>PTYPKYLLSPETIEALRKPTFDVWLWEPNEMLSCLEHMYHDLGLVRDFSINPVTLRRWLFCVHDNYRNNPFHNFRHCFCVAQMMYSMVWLCSLQEKFSQTDILILMTAAICHDLDHPGYNNTYQINARTELAVRYNDISPLENHHCAVAFQILAEPECNIFSNIPPDGFKQIRQGMITLILATDMARHAEIMDSFKEKMENFDYSNEEHMTLLKMILIKCCDISNAVRPMEVAEPWVDCLLEEYFMQSDREKSEGLPVAP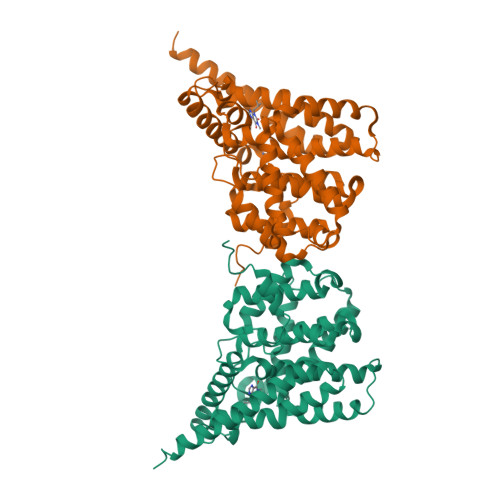FMDRDKVTKATAQIGFIKFVLIPMFETVTKLFPMVEEIMLQPLWESRDRYEELKRIDDAMKELQKK[2x]>MIHLVDYALLKPYLTVDEAVAGARKAEELGVAAYCVNPIYAPVVRPLLRKVKLCVVADFPFGALPTASRIALVSRLAEVADEIDVVAPIGLVKSRRWAEVRRDLISVVGAAGGRVVKVITEEPYLRDEERYTLYDIIAEAG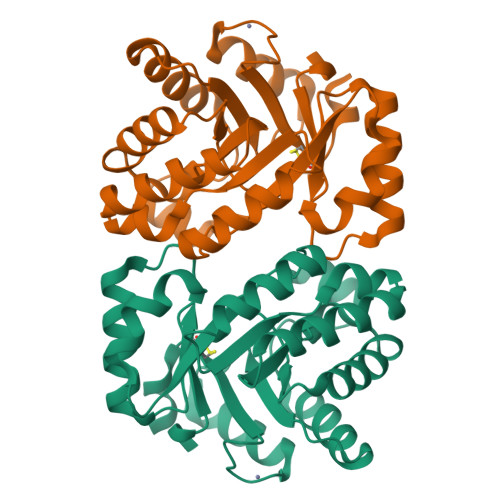AHFIKSSTGFAEEAYAARQGNPVHSTPERAAAIARYIKEKGYRLGVKMAGGIRTREQAKAIVDAIGWGEDPARVRLGTSTPEALL[2x]ethyl (R)-{10-[(hept-6-yn-1-ylcarbamoyl)oxy]decyl}phosphonofluoridate | C20 H37 F N O4 P | 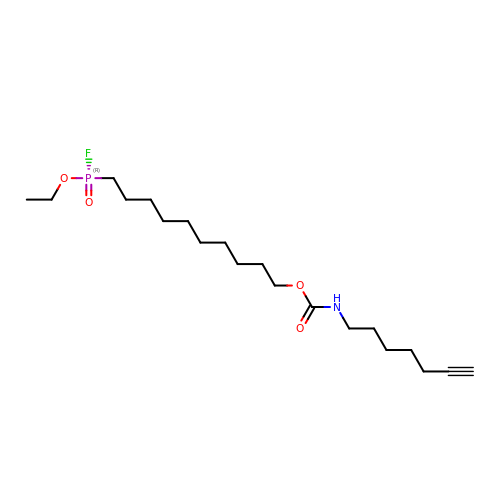JFCFPSBLBVUKMV-HHHXNRCGSA-N2-[4-(4-CHLOROPHENOXY)PHENYL]-1H-BENZIMIDAZOLE-6-CARBOXAMIDE | C20 H14 Cl 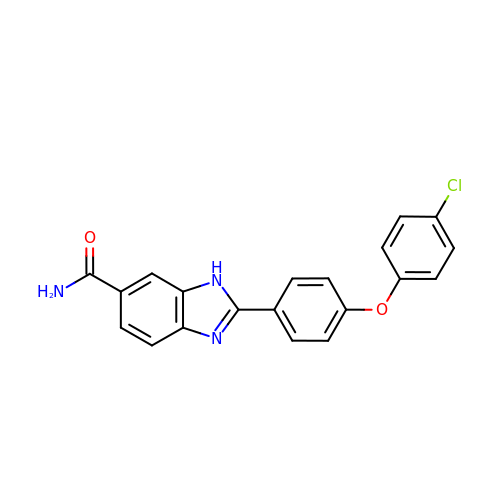N3 O2 | UXGJAOIJSROTTN-UHFFFAOYSA-N>MAHHHHHHMTHALDRFRLDGRRALITGSGRGIGLTLARGLAEAGAAIVINDRNEEKAATLARRFRDEGFAADHAVFDVAEHAQVRAAIDEFEARVGAIDILVNNAGIQRRAPLDAFEPDDWHALMRVNLDGVFNVAQAVARHMIARGHGKIINI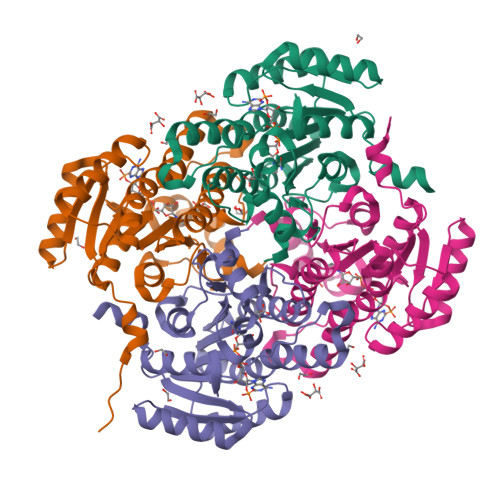CSVQSELARPTIAPYAATKGAVRMLTKGMCADWARYGIQANGLAPGYFETELNRALVDDAAFSDWLCKRTPAGRWGQVDELCGAAIFLASAASDFVNGQTLFVDGGLTSAV[4x]3-(3-acetamidophenyl)-5-quinolin-7-yl-benzoic 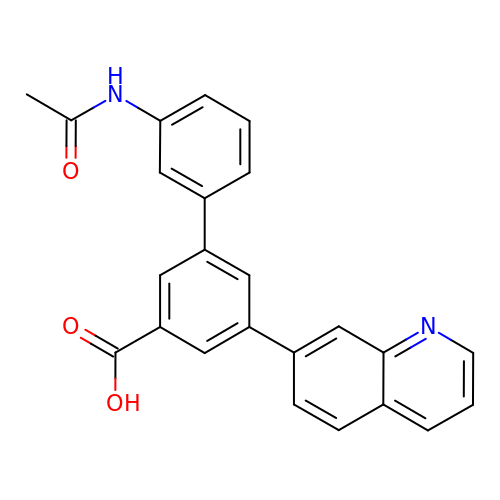acid | C24 H18 N2 O3 | HFHBEVQSZIRVAZ-UHFFFAOYSA-N> MSSRNNPARVAIVMGSKSDWATMQFAAEIFEILNVPHHVEVVSAHRTPDKLFSFAESAEENGYQVIIAGAGGAAHLPGMIAAKTLVPVLGVPVQSAALSGVDSLYSIVQMPRGIPVGTLAIGKA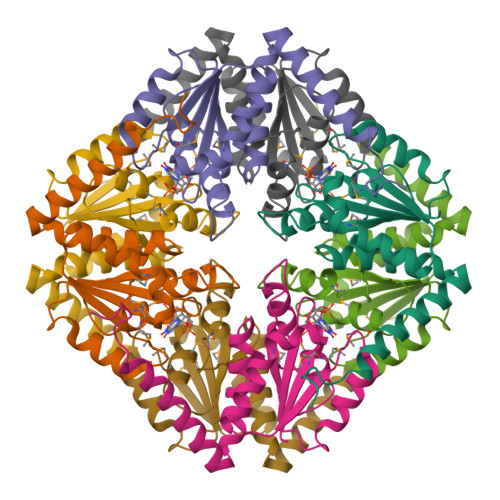GAANAALLAAQILATHDKELHQRLNDWRKAQTDEVLENPDPRGAA>MVNQVATDRFIQDLERVAQVRSEMSVCLNKLAETINKAELAGDSSSGKLSLERDIEDITIASKNLQQGVFRLLVLGDMKRGKSTFLNALIGENLLPSDVNPCTAVLTVLRYGPEKKVTIHFNDGKSPQQLDFQNFKYKYTIDPAEAKKLEQEKKQAFPDVDYAVVEYPLTLLQKGIEIVDSPGLNDTEARNELSLGYVNNCHAILFVMRASQPCTLGERRYLENYIKGRGLTVFFLVNAWDQVRESLIDPDDVEELQASENRLRQVFNANLAEYCTVEGQNIYDERVFELSSIQALRRRLKNPQADLDGTGFPKFMDSLNTFLTRERAIAELRQVRTLARLACNHTREAVARRIPLLEQDVNELKKRIDSVEPEFNKLTGIRDEFQKEIINTRDTQARTISESFRSYVLNLGNTFENDFLRYQPELNLFDFLSSGKREAFNAALQKAFEQYITDKSAAWTLTAEKDINAAFKELSRSASQYGASYNQ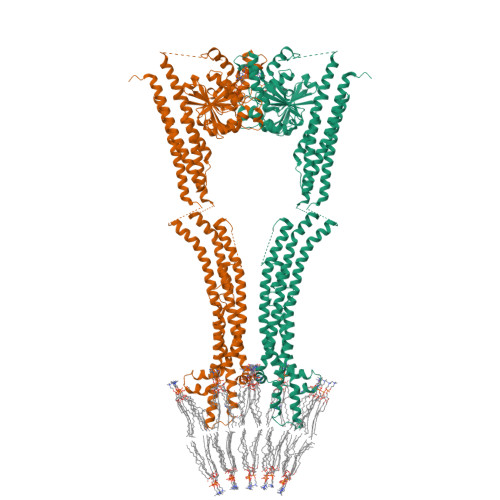ITDQITEKLTGKDVKVHTTTTAEEDNSPGWAKWAMGLLSLSKGNLAGFALAGAGFDWKNILLNYFTVIGIGGIITAVTGILLGPIGFALLGLGVGFLQADQARRELVKTAKKELVKHLPQVAHEQSQVVYNAVKECFDSYEREVSKRINDDIVSRKSELDNLVKQKQTREINRESEFNRLKNLQEDVIAQLQKIEAAYSNLLAYYSHH[2x]2-[(3,4-dichlorobenzyl)amino]ethanesulfonic 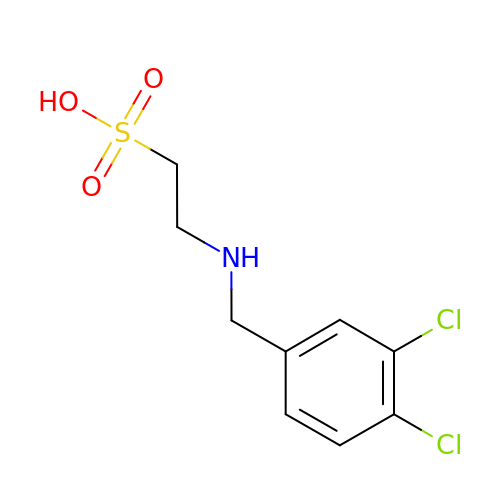acid | C9 H11 Cl2 N O3 S | MICQJBUMTVEPRD-UHFFFAOYSA-N(trans-4-{2-[(1R)-1-hydroxyethyl]imidazo[4,5-d]pyrrolo[2,3-b]pyridin-1(6H)-yl}cyclohexyl)acetonitrile | C18 H21 N5 O | 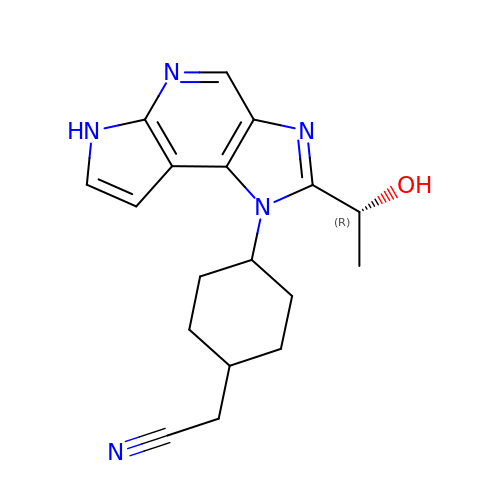IKSRDHMMQOCRHN-JHJVBQTASA-N> GAQVSRQNVGTHSTQNMVSNGSSLNYFNINYFKDAASSGASRLDFS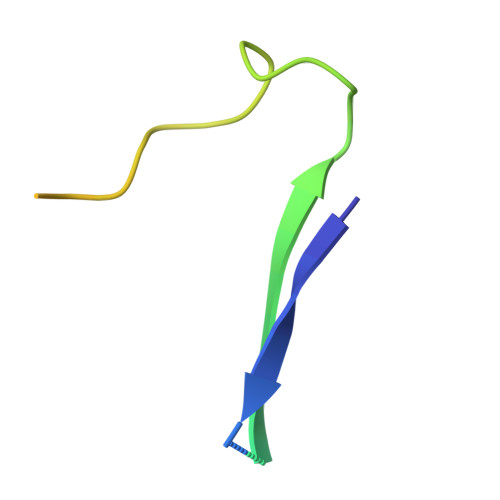QDPSKFTDPVKDVLEKGIPTLQ> MLSKRDAILKAAVEVFGKKGYDRATTDEIAEKAGVAKGLIFHYFKNKEELYYQAYMSVTEKLQKE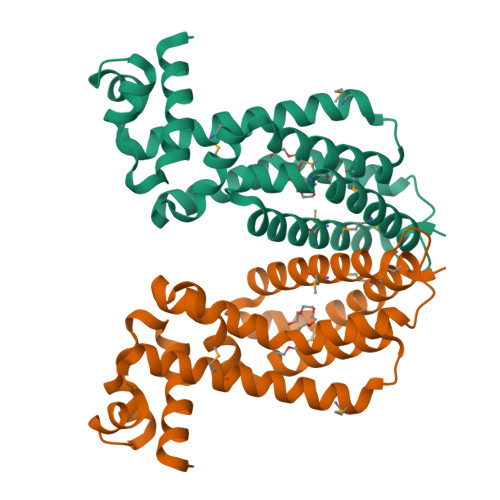FENFLMKNRNRDIFDFMERWIEKKLEYSASHPEEADFLITLVSVDEGLRKRILLDLEKSQRVFFDFVREKLKDLDLAEDVTEEIALKFLMWFFSGFEEVYLRTYQGKPELLKRDMNTLVEEVKVMLRILKKGMTK> KEQTSFNNPEPMTGFEHTVTFDFQGTKMVIPYGYLARYTQDNATKWLSDTPGQDAYSINLIEISVYYKKTDQGWVLEPYNQQNKAHFIQFLRDGLDSVDDIVIRKDACSLSTTMGERLLTYGVKKMPSAYPEYEAYEDKRHIPENPYFHEFYYIKKGENPAIITHRNNRINQTEEDSYSTSVGSCINGFTVQYYPFIREKQQLTQQELVGYHQQVEQLVQSFVNNSNKKLE

FrpD is a highly conserved lipoprotein located in the outer membrane of all meningococcal strains, and it does not exhibit similarity to known protein sequences from other organisms. Intriguingly, the FrpC1-414 fragment exhibits a very high affinity (KD ~ 0.2 nM) for FrpD, the other protein expressed from the iron-regulated frpDC operon. FrpD displays a compact, slightly concave bean-shaped structure and consists of fourteen β strands (β1–β14), one 310 helix (η1), two short α helices (α1, α2), and one long C-terminal helix α3. Hence, the similarity of FrpD fold topology to other proteins was not sufficient for establishment of structural homology, indicating that FrpD possesses a novel fold.

The FrpD43-271 protein (FrpD), a construct lacking the first 42 residues encompassing the N-terminal signal peptide (residues 1–24) and the linker sequence (residues 24–43), has been previously characterized. The protein crystallized in two alternative crystal forms, belonging to the hexagonal space group P64 and the orthorhombic space group P212121, both accommodating a single molecule in the asymmetric unit. The structure of native FrpD was determined at 2.3 Å resolution by molecular replacement using the SeMet FrpD structure and refined to an R value of 18.3% (Rfree of 24.9%). The refined crystallographic models of FrpD comprise 224 of the 229 residues, with one N-terminal and four C-terminal residues being disordered. Both FrpD structures are largely identical, with a coordinate root-mean-square deviation (rmsd) of 0.56 Å over the 224 aligned residues. The FrpD fold comprises three blocks of β sheets (I-III) flanked by helices. Block I is an antiparallel β sheet composed of the β1, β2 and β5 strands; block II contains two antiparallel β strands (β3 and β4); and block III is a nine-stranded antiparallel β sheet composed of the β6 to β14 strands. A single disulphide bond in a right-handed spiral conformation is present between the Cys150 and Cys227 residues. The electrostatic surface potential map revealed that the FrpD surface is highly negatively charged, except for a single positively charged region located at the β9 and β10 strands of the structure.> MPISPIETVPVKLKPGMDGPKVKQWPLTEEKIKALVEICTEMEKEGKISKIGPENPYNTPVFAIKKKDSTKWRKLVDFRELNKRTQDFWEVQLGIPHPAGLKKKKSVTVLDVGDAYFSVPLDEDFRKYTAFTIPSINNETPGIRYQYNVLPQGWKGSPAIFQSSMTKILEPFRKQNPDIVIYQYMDDLYVGSDLEIGQHRT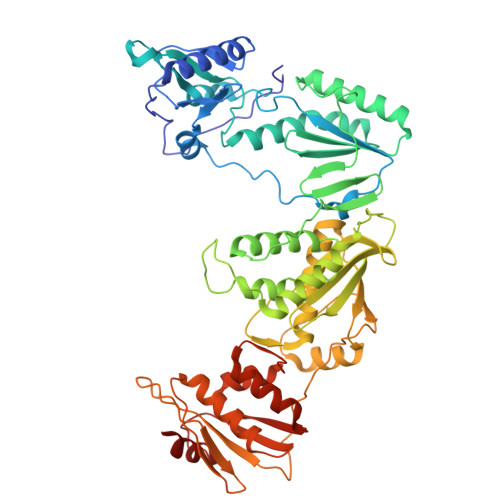KIEELRQHLLRWGLTTPDKKHQKEPPFLWMGYELHPDKWTVQPIVLPEKDSWTVNDIQKLVGKLNWASQIYPGIKVRQLCKLLRGTKALTEVIPLTEEAELELAENREILKEPVHGVYYDPSKDLIAEIQKQGQGQWTYQIYQEPFKNLKTGKYARMRGAHTNDVKQLTEAVQKITTESIVIWGKTPKFKLPIQKETWETWWTEYWQATWIPEWEFVNTPPLVKLWYQLEKEPIVGAETFYVDGAANRETKLGKAGYVTNRGRQKVVTLTDTTNQKTELQAIYLALQDSGLEVNIVTDSQYALGIIQAQPDQSESELVNQIIEQLIKKEKVYLAWVPAHKGIGGNEQVDKLVSAGIRKVL>[4x]ASGSPTGGQIVAGSGSIQTPSGNQMNIHQNSQNMVANWNSFDIGKGNTVQFDQPSSSAVALNRVVGGGESQIMGNLKANGQVFLVNPNGVLFGEGASVSTSGFVASTRDIKNDDFMNRRYT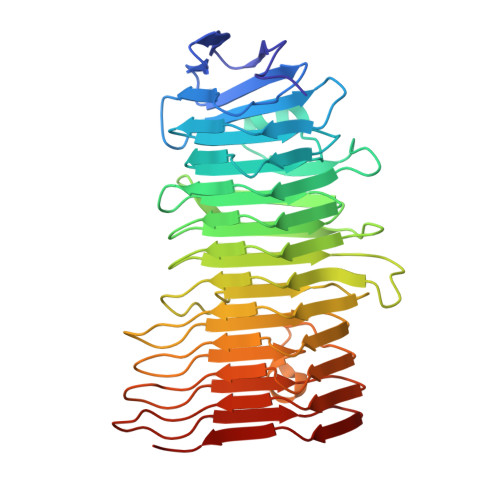FSGGQKAGAAIVNQGELTTNAGGYIVLAADRVSNSGTIRTPGGKTVLAASERITLQLDNGGLMSVQVTGDVVNALVENRGLVSARDGQVYLTALGRGMLMNTVLNVSGVVEASGMHRQDGNIVLDGGDSGVVHLSGTLQADNASGQGGKVVVQGKNILLDKGSNITATGGQGGGEVYVGGGWQGKDSNIRNADKVVMQGGARIDVSATQQGNGGTAVLWSDSYTNFHGQIGAKGGETGGNGGRVETSSHGNLQAFGTVSASAA> MPISPIETVPVKLKPGMDGPKVKQWPLTEEKIKALVEICTEMEKEGKISKIGPENPYNTPVFAIKKKDSTKWRKLVDFRELNKRTQDFWEVQLGIPHPAGLKKKKSVTVLDVGDAYFSVPLDEDFRKYTAFTIPSINNETPGIRYQYNVLPQGWKGSPAISQSSMTKILEPFKKQNPDIVIYQYMDDLYVGSDLEIGQHRTKIEELRQHLLRWGLTTPDKKHQKEPPFLWMGYELHPDKWTVQPIVLPEKDSWTVNDIQKLVGKLNWASQIYPGIKVRQLSKLLRGTKALTEVIPLTEEAELELAENREILKEPVHGVYYDPSKDLIAEIQKQGQGQWTYQIYQEPFKNLKTGKYARMRGAHTNDVKQLTEAVQKITTESIVIWGKTPKFKLPIQKETWETWWTEYWQATWIPEWEFVNTPPLVKLWYQLEKEPIVGAETFY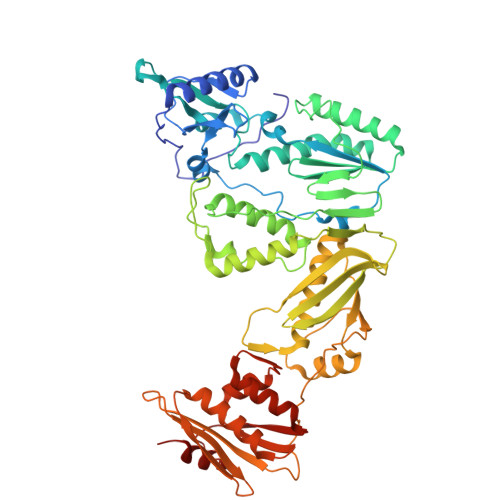VDGAANRETKLGKAGYVTNKGRQKVVPLTNTTNQKTELQAIYLALQDSGLEVNIVTDSQYALGIIQAQPDKSESELVNQIIEQLIKKEKVYLAWVPAHKGIGGNEQVDKLVSAG>[2x]MGKAVIAIHGGAGAISRAQMSLQQELRYIEALSAIVETGQKMLEAGESALDVVTEAVRLLEECPLFNAGIGAVFTRDETHELDACVMDGNTLKAGAVAGVSHLRNPVLAARLVMEQSPHVMMIGEGAENFAFARGMERVSPEIFSTSLRYEQLLAARKEGATVLDHSGAPLDEKQKMG;>TVGAVALDLDGNLAAATSTGGMTNKLPYQVGPTPLVGAGCYANNASVAVSCTGTGEVFIRALAAYDIAALMDYGGLSLAEACERVVMEKLPALGGSGGLIAIDHEGNVALPFNTEGMYRAWGYAGDTPTTGIYREKGDTVATQ[2x]

l-Asparaginases hydrolyze l-asparagine to l-aspartic acid and ammonia. The prototypic class 2 enzyme is EcAIII from E. coli. EcAIII belongs to the Ntn-hydrolases, which are expressed as immature polypeptides that dimerize and then autocatalytically cleave themselves into α (∼20 kDa) and β (∼15 kDa) subunits to form the mature (αβ)2 heterotetramer (a dimer of two αβ heterodimers). The same Thr179 acts as the nucleophile in the autoproteolytic maturation and in l-asparagine hydrolysis.

Variant RDM1-8 has two relatively large substitutions at positions 206 (Tyr) and 207 (Gln). The side chain of Tyr206 occupies the space between Glu81 and Glu125. The side chain of Gln207 is directed towards the active site, and in one dimer subunit (B) is hydrogen-bonded via water molecules to the N atoms of Leu204, Met200, Val120 and Met121, the carbonyl O atom of Val208 and the side chain (Nδ1) of His119. The nearby side chain of Glu234 is rotated towards Arg238. In contrast, in the second dimer subunit (D) Glu234 is directed towards the center of the active site and is hydrogen-bonded to the Nɛ2 atom of Gln207. The small side chain of Ala at position 207 is neutral; it does not affect the protein structure and does not participate in hydrogen bonds. In both the RDM1-8 and RDM1-24 variants the D210S/S211T substitutions are similar in their chemical character to the natural residues and support the pattern of hydrogen bonds typical of the WT protein. Similarly, in our variant RDM1-8 the R207Q mutation did not abolish autocleavage.>[3x]MWLRAFILATLSASAAWGHPSSPPVVDTVHGKVLGKFVSLEGFAQPVAIFLGIPFAKPPLGPL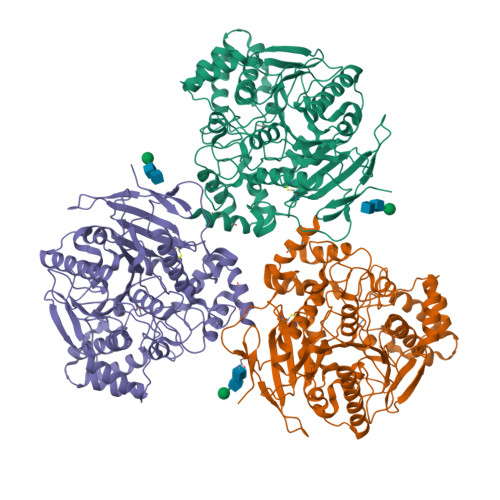RFTPPQPAEPWSFVKNATSYPPMCTQDPKAGQLLSELFTNRKENIPLKLSEDCLYLNIYTPADLTKKNRLPVMVWIHGGGLMVGAASTYDGLALAAHENVVVVTIQYRLGIWGFFSTGDEHSRGNWGHLDQVAALRWVQDNIASFGGNPGSVTIFGESAGGESVSVLVLSPLAKNLFHRAISESGVALTSVLVKKGDVKPLAEQIAITAGCKTTTSAVMVHCLRQKTEEELLETTLKMKFLSLDLQGDPRESQPLLGTVIDGMLLLKTPEELQAERNFHTVPYMVGINKQEFGWLIPMQLMSYPLSEGQLDQKTAMSLLWKSYPLVCIAKELIPEATEKYLGGTDDTVKKKDLFLDLIADVMFGVPSVIVARNHRDAGAPTYMYEFQYRPSFSSDMKPKTVIGDHGDELFSVFGAPFLKEGASEEEIRLSKMVMKFWANFARNGNPNGEGLPHWPEYNQKEGYLQIGANTQAAQKLKDKEVAFWTNLFAKKAVEKPPQTEHIEL We report an in silico strategy for the biocatalytic synthesis of chiral N- and O-heterocycles via Baldwin cyclization modes of hydroxy- and amino-substituted epoxides and oxetanes using the limonene epoxide hydrolase from Rhodococcus erythropolis. We turned to cofactor-independent limonene epoxide hydrolases (LEHs) that normally catalyze direct hydrolysis of epoxides by positioning and activating water at the active site. On the basis of the well-documented mechanism of ReLEH, a water molecular is positioned by H-bonds to N55 and Y53 while D132 abstracts a proton from the water, enabling a smooth nucleophilic attack on one of the substrate’s epoxide carbon center. We have rationally engineered the epoxide hydrolase ReLEH with construction of a general platform for Baldwin cyclization reactivity of hydroxy- and amino-epoxides and oxetanes.

To further elucidate the mechanism, crystallographic experiments were performed. We obtained the complex crystals of SZ611-substrate 59 and SZ611-product 46 using the soaking methods as described in Material and Methods. SZ611 assembles into a homodimer structure with four α-helices and five-strand β-sheets in each monomer, forming a cavity that serves as a deep substrate-binding pocket, in which a substituent of substrate 59 or of product 46 can occur without steric repulsion. In contrast, product 46 was well-defined in the electron density map, including the phenyl group corresponding to that of substrate 59. The phenyl group is located in the hydrophobic local space formed by the hydrophobic residues of L71, L74 and F75, which were clearly defined in the electron density map. Two other essential mutations, Y53F and N55A, have well-defined electron density maps that together expand the hydrophobic local space, thereby leading to the preference of intramolecular cyclization reactions. The molecular architecture of substrate 46 in the binding pocket was mainly attributed to its multiple interactions with catalytic residues D101 and D132. Product 46 shares a similar conformation with substrate 59 considering the hydrogen-bonding networks of amines and hydroxyl groups with D132 and D101, which together predicts a pathway for the LEH-catalyzed selective desymmetrization reactions of oxetanes. In the catalytic reactions, residue D132 acts as a proton acceptor to promote the deprotonation of the amino group. The deprotonated N-atom then nucleophilically attacks the oxetane moiety, resulting in ring opening, followed by the protonation of the O-atom of the oxetane precursor with D101 as the proton donor.

>MHHHHHHTSKIEQPRWASKDSAAGAASTPDEKIVLEFMDALTSNDAAKLIEYFAEDTMFQAMPLPPAYGRDAVEQTLAGLFTVMSIDAVETFHIGSSNGLVYTERVDVLRALPTGKSYNLSILGVFQLTEGKITGWRDYFDLREFEEAVDLPLRG[4x]> KVLKISQTKYEEILKISKKYIFINQVDKSFHEAVDDLNQQDFIAVSGDGANMGRKCKMPFLVLSTDHQIYIFDIQVMQYHAFESGLKKILEGDSPKKIAHDCRKLSDCLYHKHNVKLKSVFDTQVGDLIITKNKKVTLPNKVKSLGECLTNYLGLQQNTIDEKLDIVQSTERPLSVKIKDSLARNIAFLHHLSEVINEEMQLPFYRGVECYIENIRSSDDFKAWELCGKLNQIPKEFRNAIDY;> KVLKISQTKYEEILKISKKYIFINQVDKSFHEAVDDLNQQDFIAVSGDGANMGRKCKMPFLVLSTDHQIYIFDIQVMQYHAFESGLKKILEGDSPRKIAHDCRKLSDCLYHKHNVKLKSVFDTQVGDLIITKNK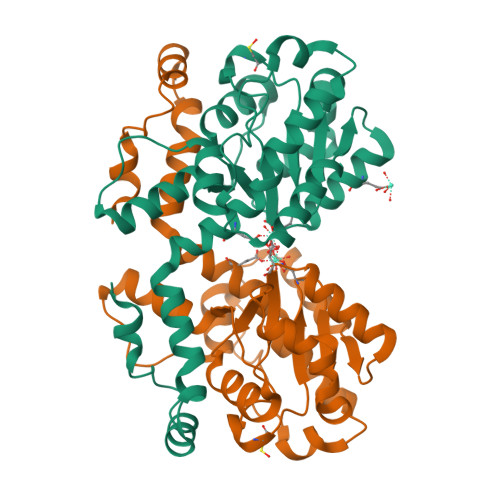KVTLPNKVKSLGECLTNYLGLQQNTIDEKLDIVQSTERPLSVKIKDSLARNIAFLHHLSEVINEEMQLPFYRGVECYIENIRSSDDFKAWELCGKLNQIPKEFRNAIDY Legionella pneumophila, the causative agent of Legionnaires disease, secretes the enzyme AnkX that uses cytidine diphosphate-choline to post-translationally modify the human small G-Protein Rab1 with a phosphocholine moiety at Ser76. Later in the infection, the Legionella enzyme Lem3 acts as a dephosphocholinase, hydrolytically removing the phosphocholine. Through crystal structures of Lem3 in the apo form and in complex with Rab1b, we reveal Lem3’s catalytic mechanism, showing that it acts on Rab1 by locally unfolding it. Since Lem3 shares high structural similarity with metal-dependent protein phosphatases, our Lem3:Rab1b complex structure also sheds light on how these phosphatases recognise protein substrates.

In order to obtain structural insights into Lem3, we crystallised the full-length protein comprising the amino acids (aa) 1-570 (Lem3FL) and a shortened construct (aa 21-486, Lem321-486). We solved the structures of Lem3FL and Lem321-486 at 3.6 Å and 2.2 Å resolution, respectively. Lem321-486 differs from the conserved PPM1A fold in minor details: The central β-sheet core consists of two additional β-strands (β1 and β19), thereby broadening the cleft. The spatial orientation of the additional α-helices forming the thumb shape a deep cavity located at the interception of the fist and the thumb (referred to as the hollow region). The base of this hollow region, which is located closely to the β-sheet cleft in the active centre, harbours the metal ions. As verified by CheckMyMetal, these metal ions are embedded in an octahedral cluster which is characteristic of the coordination of Mg2+, Mn2+, or Ca2+ ions. This metal cluster is surrounded by a scaffold of oxygen atoms provided by the side chains of four aspartate residues (D82Lem3, D105Lem3, D254Lem3, and D394Lem3), the backbone carbonyl of a glycine (G106Lem3) as well as six water molecules. More precisely, M1 is coordinated by D105Lem3, D254Lem3, D394Lem3, and three water molecules. M2 is coordinated by D105Lem3, the main chain-oxygen atom of G106Lem3, and four solvent molecules. Additionally, the effect of the mutation of D190Lem3 was examined since it is located in close proximity to the metal ions, suggesting that it could be involved in their coordination.

>[4x]GHDKIITGKKIIFSQSVAKDQTKNLSSFLSERFYSVNQSHNHSIIIGSSLSHQENDIEHDTILDTSGVLVTTDTNGIVNGARVAITDGLGGGNGDQEEDDEIYRVSHSSCENFLNCDQNIDTTLSLITQPKASDKKQTAPKTLQHTEASMAAFIYQNHPGKGYIGEFANIGAGLIIILDKRFKIKHMVSACHIYRGFGTWTPPSLQALATTANKDALLVRQTLKLAEGDIIISMTDGVWGELKTSLIAQTNDRRDIGVDKEYFKTLFDELTDAPYPSSFDIARIITQRAMSRSLERRKTLIKLINEIEQQHFHEKSVKTINEVLEYFIKTGHVETAQTLKAILFEDGLSDGITYFENIEIPLEMVMHDLKSRTVGDCSTINVTRIPYHLDELIRGFINYPEKHQILAPLFKARVKSEADLEEAFHRLSLEMVQPEIECPISETHFERAFKKETLDKTQAVLTHYFRIS> HMILKCILAFLLMVNEGWKMKILVRNLDRSVTEAEVLELFKAYG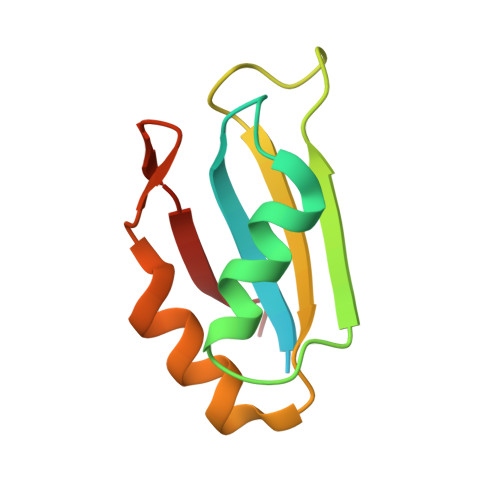KVESCVVVTDKDTGKSKGFGFVEMPNPREAIKAIKGLNTLKVKGYGIRVKAAEE>MSKSDVFHLGLTKNDLQGAQLAIVPGDPERVEKIAALMDKPVKLASHREFTSWRAELDGKAVIVCSTGIGGPSTSIAVEELAQLGIRTFLRIGTTGAIQPHINVGDVLVTTASVRLDGASLHFAPMEFPAVADFACTTALVEAAKSIGATTHVGVTASSDTFYPGQERYDTYSGRVVRRFKGSMEEWQAMGVMNYEMESATLLTMCASQGLRAGMVAGVIVNRTQQEIPNAETMKQTESHAVK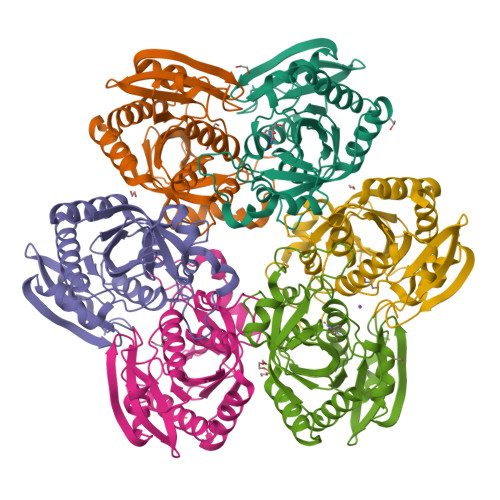IVVEAARRLL[6x]> KKEPEGL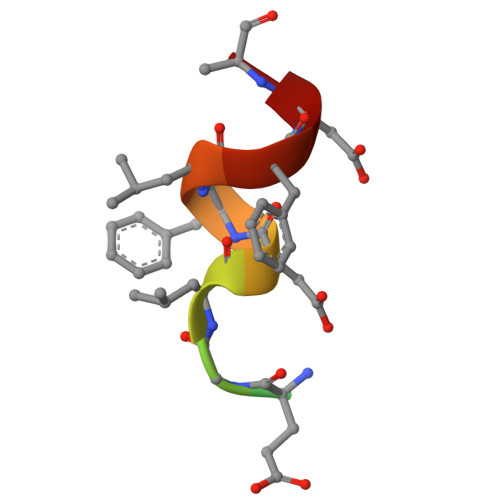DFLFDA[7-azanyl-10-[5-[2-[2-(6-chloranylhexoxy)ethoxy]ethylcarbamoyl]-2-(cyanocarbamoyl)phenyl]-5,5-dimethyl-benzo[b][1]benzosilin-3-ylidene]-methyl-azanium 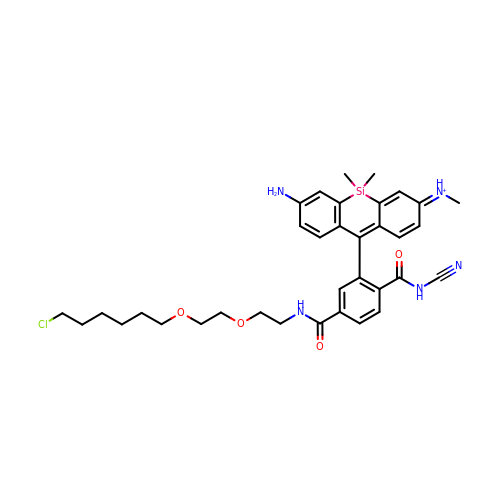| C35 H43 Cl N5 O4 Si | MOOPIZWXYFKFBC-JBFMKSPFSA-O> MLRARRPLPLLPGSRAWLLRFYSSTRELCQLQSRERLILGTHGAGVVQHASVSQPLSVNFQSSVTVAAPAADLFRTKVHEGTGTSGKDPYLRTLPNQESREPESSVSQAHITVAPTVDECSTLDRRWESMQYWFNDQHPRLVIYLRQLQVQDVPPISPAAESLLSKFEEVAIPKLALDDTDRQRLTKLWGNLTEEAKALRLHYVFDRFAFESKLSQLCKEALEQMHAMSLSGTEGSLAVEALRRLTILKRNDYIQRHLIDVTSNGAYLGFGDAVWRVFFSAVEAHKAVLFGKGTPDTIRFAWESILQEDVVRVPDVTAPVALFLTLVCIHEGNRLASVEWRESSSSLDEGICSSDNTQQRPLLALLNPVVKRRFVTKMVEFLLRSHSSNEFSKLLRKHGLHDLSRDVALCEAMNGSQGILEDDVAELVSRFESTGEVKTLLSSLIGGKDAAVRETVAKIMGIPLATTVDWDAMMQSVDWTNNWRRLATKLLCDQTLLVSIHKLVKNAIGAKGISR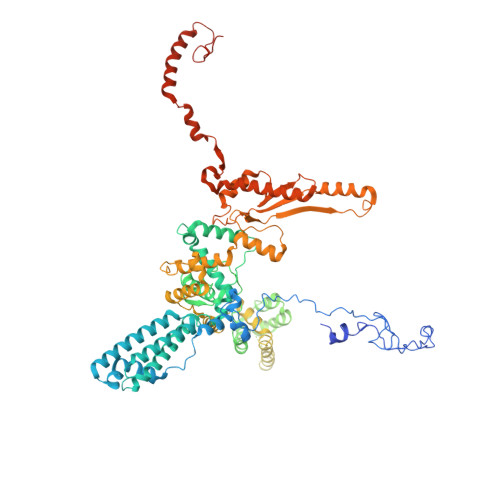HLFSEEYADQLQSIIAIREERELNRKLKIDRIVRELSSYQRVDQSCEMLRQLGVDMKELDQAALSIRQDGLVKRPSVDENVISRALEAVGNRHPNWVRAGVIAPGAIKDSIGALKAMLFIFIRLSYVPQTGLAAMAQRFRRRIGPIGVESFQFNIPTEVGFVEHYNNLEYKRYDWQGWYQRMVDVHNRNISLRCRVSDLKRLDPNGVPFVDMQTERRLRILAEGRVGMGVLMLDSDKYEDQKDNMTFGSIKLSELLSDARKAQLGEEYWPSVEMKVRKPSGQSKAHYSLIDYDRIEKKSRELYEKYRDAKKKSLFVTPMDLWLEVKGMQVRKASDGADADGYTVDILQDALSSEDNEKH> MAISIKTPEDIEKMRVAGRLAAEVLEMIEPYVKPGVSTGELDRICNDYIVNEQHAVSACLGYHGYPKSVCISINEVVCHGIPDDAKLLKDGDIVNIDVTVIKDGFHGDTSKMFIVGKPTIMGERLCRITQESLYLALRMVKPGINLREIGAAIQKFVEAEGFSVVREYCGHGIGQGFHEEPQVLHYDSRETNVVLKPGMTFTIEPMVNAGKKEIRTMKDGWTVKTKDRSLSAQYEHTIVVTDNGCEILTLRKDDTIPAIISHDE;> MEVKELERDKNRVVLEYVFGAEEIAQAEDKAVRYLNQRVEIPGFRKGRIPKNVLKMKLGEEFQEYTLDF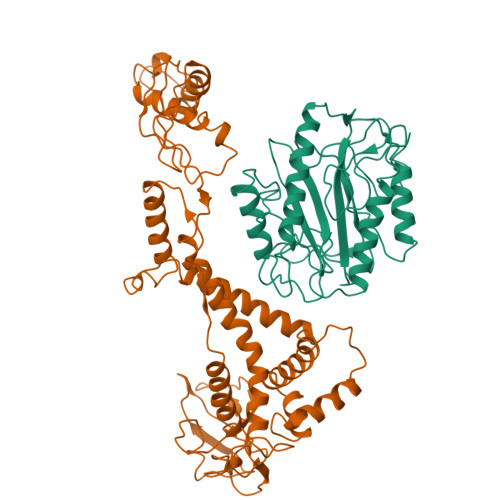LMDLIPDTLKDRKLILSPIVTERELKDVTARVVVEVHEEPEVRIGDISKIEVEKVDEEKVLEKYVERRIEDLRESHALLEPKEGPAEAGDLVRVNMEVYNEEGKKLTSREYEYVISEDEDRPFVKDLVGKKKGDVVEIEREYEGKKYTYKLEVEEVYKRTLPEIGDELAKSVNNEFETLEQLKESLKKEGKEIYDVEMKESMREQLLEKLPEIVEIEISDRTLEILVNEAINRLKREGRYEQIVSSYESEEKFREELKERILDDIKRDRVIEVLAQEKGISVNDEELEKEAEELAPFWGISPDRAKSLVKARQDLREELRWAILKRKVLDLLLQEVE> GTGPDKLKKVLDKLRLKRKDISEAAETVNKVVERLLRRMQKRESEFKGVEQLNTGSYYEHVKISAPNQFNVMFKLEVPRIELQEYYETGAFYLVKFKRIPRGNPLSHFLEGEVLSATKMLSKFRKIIKEEVKEIKDIDVSVEKEKPGSPAVTLLIRNPEEISVDIILALESKGSWPISTKEGLPIQGWLGTKVRTNLRREPFYLVPKNAKDGNSFQGETWRLSFSHTEKYILNNHGIEKTCCESSGAKCCRKECLKLMKYLLEQLKKEFQELDAFCSYHVKTAIFHMWTQDPQDSQWDPRNLSSCFDKLLAFFLECLRTEKLDHYFIPKFNLFSQELIDRKSKEFLSKKIEYERNNGFPIFDKL

Cyclic GMP-AMP (cGAMP) synthase (cGAS) is essential for the host defense against cytosolic double-stranded (ds)DNA arising from various maladies (e.g., pathogen invasion, ionizing irradiation, and genotoxic chemicals). Upon directly binding to and dimerizing on dsDNA, cGAS cyclizes ATP and GTP into 2′−5′/3′−5′-linked cGAMP, a unique metazoan second messenger for initiating type-I interferon (IFN-I)-mediated inflammatory responses. cGAS is central to antitumor immunity, host defense against an array of pathogens, and regulating autoimmunity. Here, we resolve these numerous fundamental mechanistic questions in innate immunology and present a unifying catalytic mechanism of cGAS. Finally, we reveal how mouse cGAS achieves more stringent substrate selectivity and higher catalytic efficiency than the human enzyme. Together, we set forth a unifying catalytic mechanism of cGAS in which dsDNA-binding pre-organizes the active site into a rigid yet adaptable lock for two sets of keys (substrates and intermediate) necessary to specifically synthesize 2′−5/3′−5′-cGAMP.

Moreover, soaking ATP to QN-mcGAScat crystallized with and without dsDNA showed the productive (one Mg2+) and nonproductive (no Mg2+) binding states seen from WT ± dsDNA (two Mg2+ and no Mg2+), respectively. These observations corroborate that the QN mutant is well-suited for delineating how dsDNA regulates substrate binding.Fig. 2 dsDNA regulates productive vs. nonproductive substrate binding.>MSLPMLQVALDNQTMDSAYETTRLIAEEVDIIEVGTILCVGEGVRAVRDLKALYPHKIVLADAKIADAGKILSRMCFEANADWVTVICCADINTAKGALDVAKEFNGDVQIQLTGYWTWEQAQQWRDAGIGQV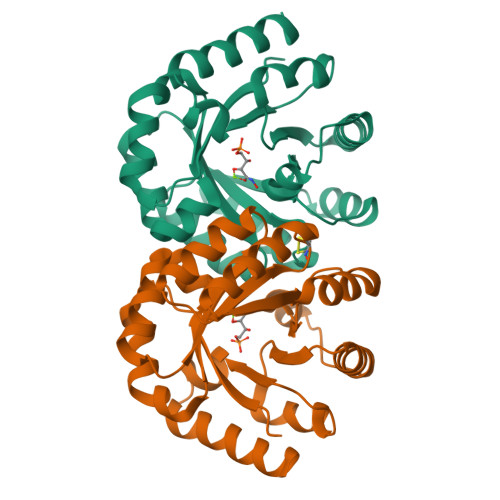VYARSRDAQAAGVAWGEADITAIKRLSDMGFKVTVTGGLALEDLPLFKGIPIHVFIAGRSIRDAASPVEAARQFKRSIAELWG[2x]>SHEQFRAALQLVVDPG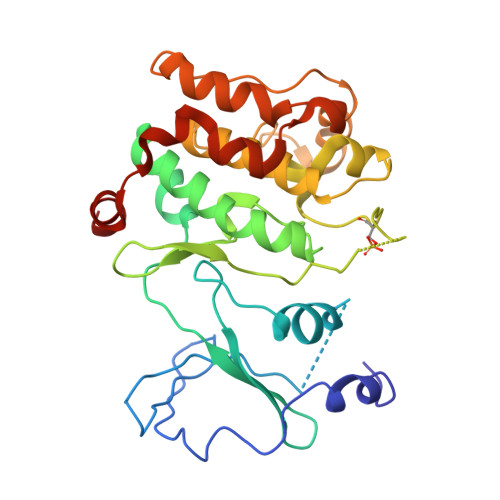DPRSYLDNFIKIGEGSTGIVCIATVRSSGKLVAVKKMDLRKQQRRELLFNEVVIMRDYQHENVVEMYNSYLVGDELWVVMEFLEGGALTDIVTHTRMNEEQIAAVCLAVLQALSVLHAQGVIHRDIKSDSILLTHDGRVKLSDFGFCAQVSKEVPRRKSLVGTPYWMAPELISRLPYGPEVDIWSLGIMVIEMVDGEPPYFNEPPLKAMKMIRDNLPPRLKNLHKVSPSLKGFLDRLLVRDPAQRATAAELLKHPFLAKAGPPASIVPLMRQNRTR[2x]>GDQPVINFGIISTESSQNLKSIWEPFLKDMSQQTGYQVKAFFAPDYAGIIQGMRFDKVDIAWYGNKAAMEAVDRAHGEIFAQTVAASGAPGYWSLLIANKDSKIDSLEDMLANAKSLTFGNGDPNS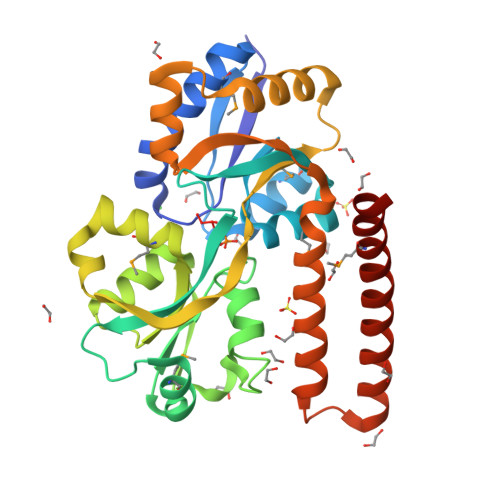TSGYLVPGYYVFAKNNVDPVKAFKRTLNSSHEVNALAVANKQVDVATFNTEGMERLELTQPEKARQLKVIWKSPLIPGDPLVWRNNLSDEQKNKLRDFFFKYGANAEQKKVLADLQWSKFQASDDDQLLPIRQLELFKQRTDVANNANLGAEEKAAKLKALDEELAKLEKRMAEREQKTAANAG[2x]>[8x]MPKKTIYFGAGWRTDRQNKAYKEAMEALKENPTIDLENSYVPLDNQYKGIRVDEHPEYLHDKVWATATYNNDLNGIKTNDIMLGVYIPDEQGTGLGMELG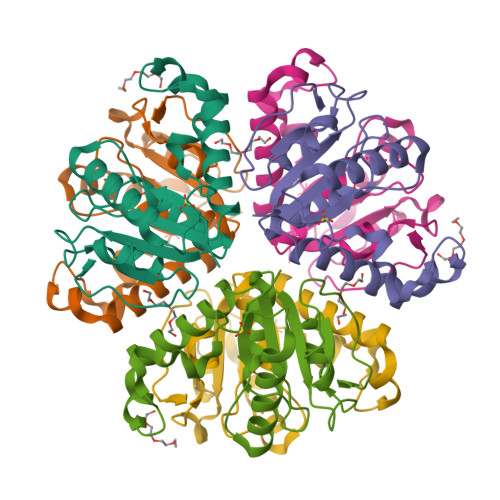YALSQGKYVLLVIPDEDYGKPISLMSWGVSDNVIKMSQLKDFNFNKPRFDFYEGAVY> SRANDAPIVLLHGFTGWGREEMFGFKYWGGVRGDIEQWLNDNGYRTYTLAVGPLSSNWDRACEAYAQLVGGTVDYGAAHAAKHGHARFGRTYPGLLPELKRGGRIHIIAHSQGGQT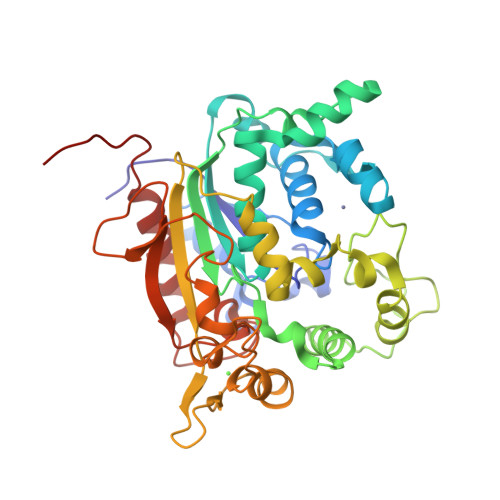ARMLVSLLENGSQEEREYAKAHNVSLSPLFEGGHHFVLSVTTIATPHDGTTLVNMVDFTDRFFDLQKAVLKAAAVASNVPYTSQVYDFKLDQWGLRRQPGESFDQYFERLKRSPVWTSTDTARYDLSVPGAEKLNQWVKASPNTYYLSFATERTYRGALTGNYYPELGMNAFSAVVCAPFLGSYRNATLGIDDRWLENDGIVNAFSMNGPKRGSTDRIVPYDGTIKKGVWNDMGTYNVDHLEVIGVDPNPLFDIRAFYLRLAEQLASLQPHHHHHH>[2x]SVCKGV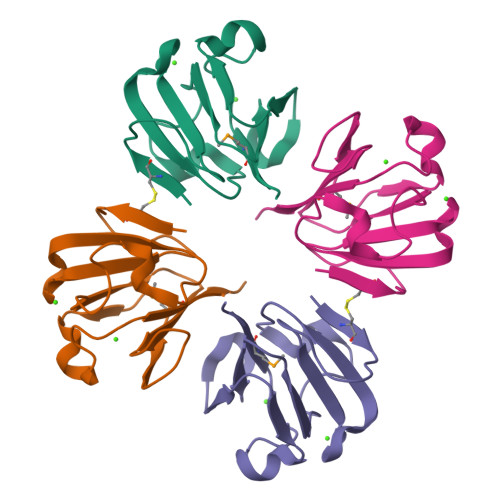SGNPAKGEVFLYKHVNFQGDSWKVTGNVYDFRSVSGLNDVVSSVKVGPNTKAFIFKDDRFNGNFIRLEESSQVTDLTTRNLNDAISSMIVATFESA>MSETPLLDELEKGPWPSFVKEIKKTAELMEKAAAEGKDVKMPKGARGLLKQLEISYKDKKTHWKHGGIVSVVGYGGGVIGRYSDLGEQIPEVEHFHTMRINQPSGWFYSTKALRGLCDVWEKWGSGLTNFHGSTGDIIFLGTRSEYLQPCFEDLGNLEIPFDIGGSGSDLRTPSACMGPALCEFACYDTLELCYDLTMTYQDELHRPMWPYKFKIKCAGCPNDCVASKARSDFAIIGTWKDDIKVDQEAVKEYASWMDIENEVVKLCPTGAIKWDGKELTIDNRECVRCMHCINKMPKALKPGDERGATILIGGKAPFVEGAVIGWVAVPFVEVEKPYDEIKEILEAIWDWWDEEGKFRERIGELIWRKGMREFLKVIGREADVRMVKAPRNNPFMFFEKDELKPSAYTEELKKRGMW[2x];>MVVEGVKTDFGPPYFRDLLHPVIAKNYGKWKYHEVVKPGVIKRVAESGDVIYVVRFGTPRLLSIYTVRELCDIADKYSDGYLRWTSRNNVEFFVTDESKIDDLINEVQERVGFPCGGTWDAVKGEYGLSNIVHTQGWIHCHTPAIDASGIVKAVMDELYEYFTDHKLPAMCRISLACCANMCGAVHASDIAIVGIHRTPPIPNDEAIRKTCEIPSTVAACPTGALKPDMKNKTIKVDVEKCMYCGNCYTMCPGMPLFDPENDGAAIMVGGKLSEARRMPELSKVVVPWVPNEPPRWPTLVKYVKQILEAWAANANKHERLIEWVDRIGWERFFELTGLEFTQHLIDDYRITPYFYSEFRASTQFKW[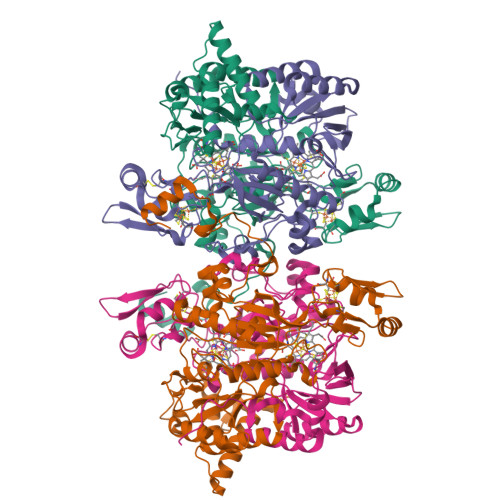2x]N-[2-(dodecanoylamino)ethyl]-N~3~-[(2R)-2-hydroxy-3,3-dimethyl-4-(phosphonooxy)butanoyl]-beta-alaninamide 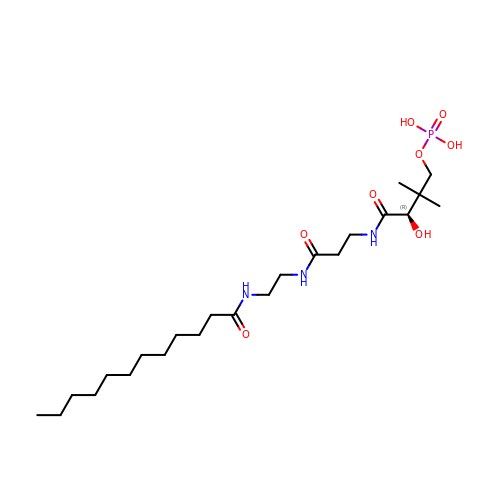| C23 H46 N3 O8 P | HNUNEXIROQFTBE-NRFANRHFSA-N> TVIKNETGTISISQLNKNVWVHTELGSFNGEAVPSNGLVLNTSKGLVLVDSSWDDKLTKELIEMVEKKFQKRVTDVIITHAHADHIGGIKTLKERGIKAHSTALTAELAKKNGYEEPLGDLQTV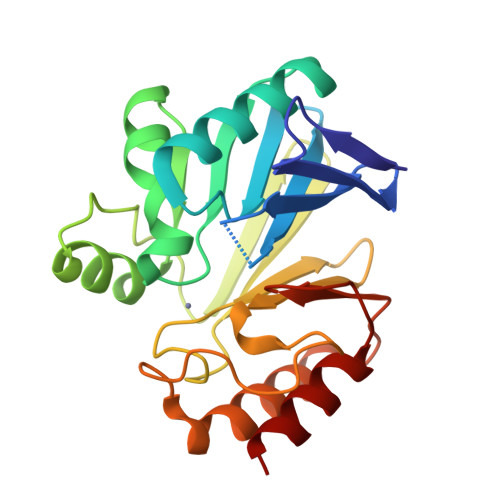TNLKFGNMKVETFYPGKGHTEDNIVVWLPQYNILVGGSLVKSTSAKDLGNVADAYVNEWSTSIENVLKRYRNINAVVPGHGEVGDKGLLLHTLDLLK> ALEGTEFARSEGASALASVNPLKTTVEEALS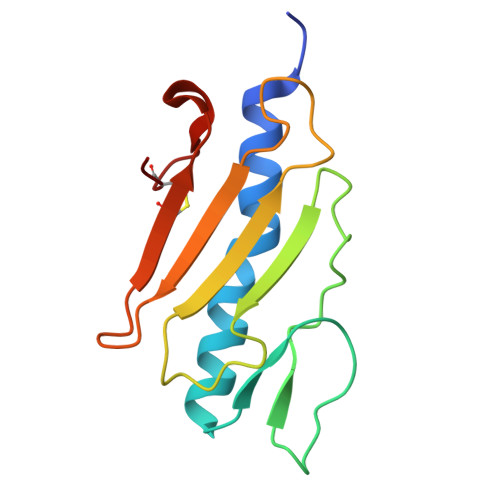RGWSVKSGTGTEDATKKEVPLGVAADANKLGTIALKPDPADGTADITLTFTMGGAGPKNKGKIITLTRTAADGLWKCTSDQDEQFIPKGCSR>KTCENLADTFRGPCFTDGSCDDHCKNKEHLIKGRCRDDF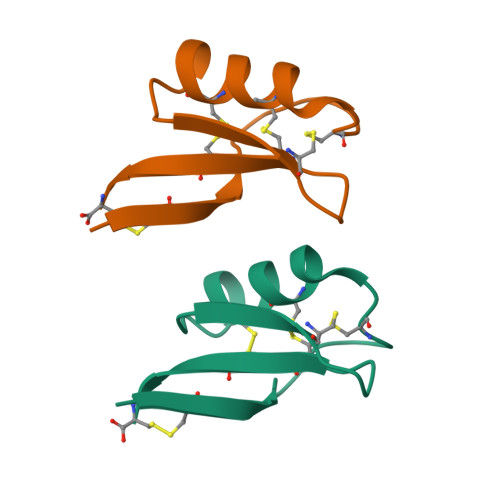RCWCTRNC[2x]2-amino-6-(methylamino)-5-nitrosopyrimidin-4(3H)-one 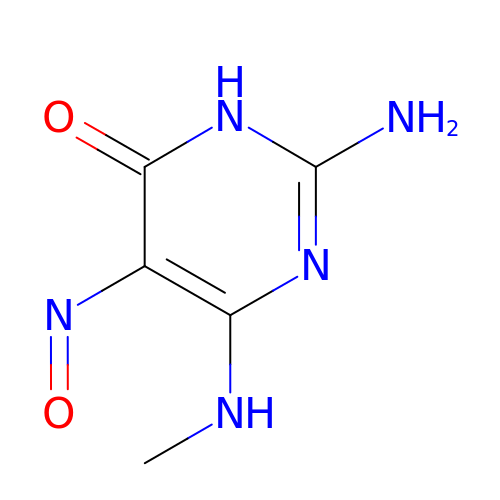| C5 H7 N5 O2 | ISOZZGJCVBHMSM-UHFFFAOYSA-N> MSAKDERAREILRGFKLNWMNLRDAETGKILWQGTEDLSVPGVEHEARVPKKILKCKAVSRELNFSSTEQMEKFRLEQKVYFKGQCLEEWFFEFGFVIPNSTNTWQSLIS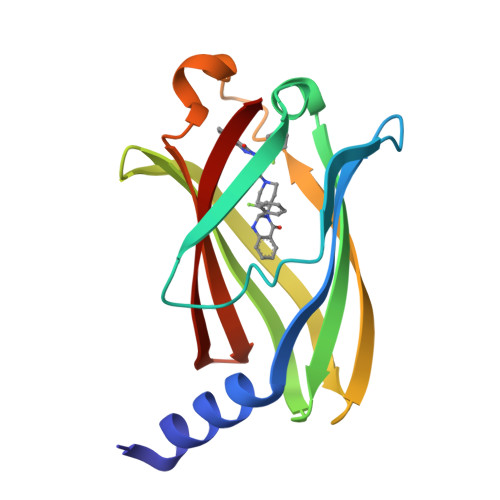AAPESQMMPASVLTGNVIIETKFFDDDLLVSTSRVRLFYV> EAIQTRAVINQHGTSETLVENFLGRAALVMMKDFEYKNHVTGTQKVQQNFFKWTINTR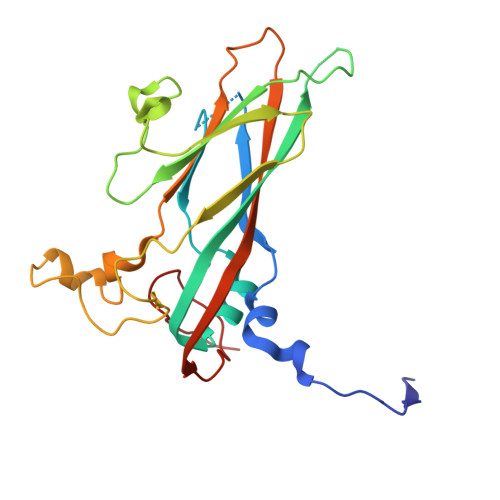SYVQLRRKFELFTYIRFDSEITIVPTIRLYTSTGASYSGLPNLTLQAMFVPVGAPTPKSQDSYEWQSACNPSVFFKIDDPPARMTIPFMCINSAYGMFYDGFAGFEKTANGLYGINPANTMGNLCIRVVNAYQPVQYTITIRIYLKPKHIKAWVPRPPRTMPYMSIANTNYTGH>[2x]MQIGIIGLGRMGGNIAVRLSRHGHDVVLFDRDAATVSKVSERIEGGRGVAATSLPDLVAKLTAKRKIVWVMLPCGEITENAVQELYGLLGKDDIVIDGGNTYYKDDIRRAAQLADKGIHYVDVGTSGGVWGLERGYCMMYGGTKDSTDHIDPILDALAPGKGDVAPTPDRGKPGLDPRAEKGYLHCGPAGSGHFVKM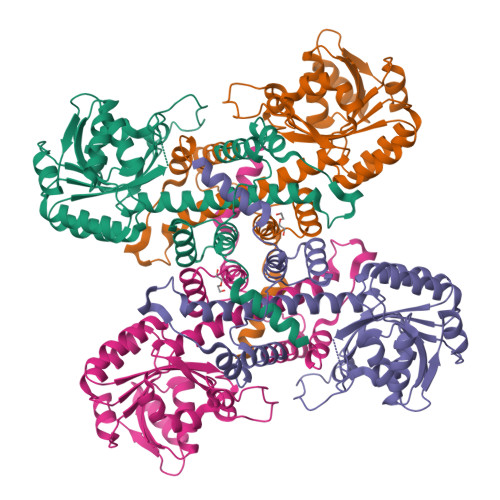VHNGIEYGMMQAFAEGFDIMKSKNSPKLPEDQRFDLNMADIAEVWRRGSVVSSWLLDLTAEALAKNASLSEFTGEVADSGEGRWTLEAAIEEAVPAPVITASLFTRFRSRTGNNYAEKVLSAMRFGFGGHVEKKD(2R,3S,4S)-5-({[(acetylcarbamoyl)amino]methyl}[(3S,4R)-6-amino-3,4-dimethylhexyl]amino)-2,3,4-trihydroxypentyl 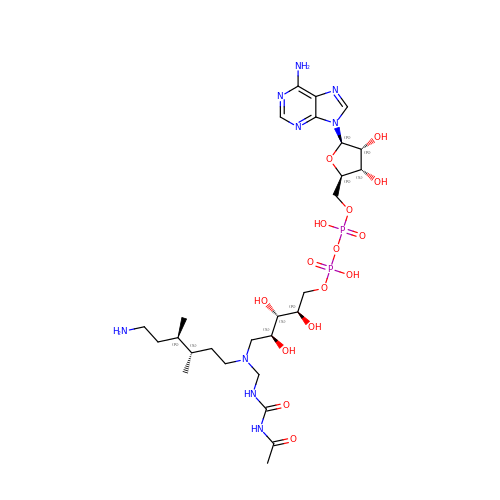[(2R,3S,4R,5R)-5-(6-amino-9H-purin-9-yl)-3,4-dihydroxytetrahydrofuran-2-yl]methyl dihydrogen diphosphate (non-preferred name) | C27 H49 N9 O15 P2 | GXAQOPQBDYJNIO-CCGDWWFSSA-N> NGEPDIAQLKGLSPSQRQAYAVQLKNRGNHFFTAKNFNEAIKYYQYAIELDPNEPVFYSNISACYISTGDLEKVIEFTTKALEIKPDHSKALLRRASANESLGNFTDAMFDLSVLSLNGDFDGASIEPMLERNLNKQAMKVLNENLSKDEGRGSQVLPSNTSLASFFGIFDSHLEVSSVNTSSNYDTAYALLSDALQRLYSATDEGYLVANDLLTKSTDMYHSLLSANTVDDPLRENAALALCYTGIFHFLKNNLLDAQVLLQESINLHPTPNSYIFLALTLADKEN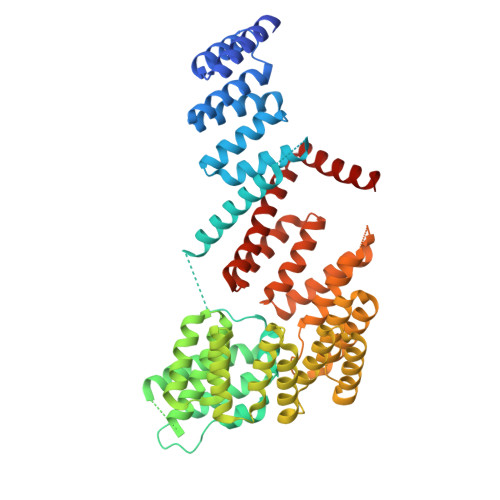SQEFFKFFQKAVDLNPEYPPTYYHRGQMYFILQDYKNAKEDFQKAQSLNPENVYPYIQLACLLYKQGKFTESEAFFNETKLKFPTLPEVPTFFAEILTDRGDFDTAIKQYDIAKRLEEVQEKIHVGIGPLIGKATILARQSSQDPTQLDEEKFNAAIKLLTKACELDPRSEQAKIGLAQLKLQMEKIDEAIELFEDSAILARTMDEKLQATTFAEAAKIQKRLRADPIISAKMELTLARYRAKGML> MDIRRLILAFILPPAAVMNKEAGTIMLTGILTLWG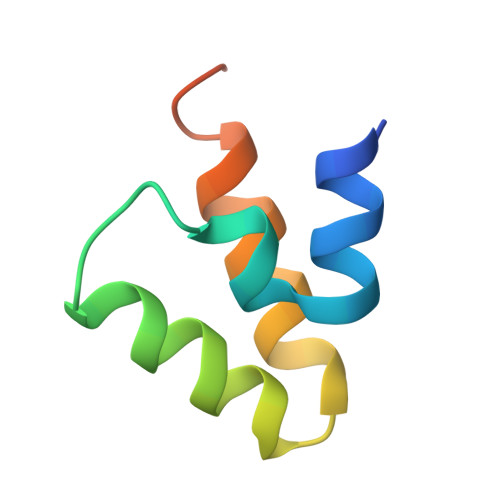WIPGVVAALIMISKEQSGKTAEA> LDHLHAAEAAYQIESIIKTATDTVKSEINAELGVVPSLNAVETGATSNTEPEEAIQTRTVINQHGVSETLVENFLSRAALVSKRSFEYKDHTSSTARADKNFFKWTINTRSFVQLRRKLELFTYLRFDAEITILTTVAVNGSGNNTYVGLPDLTLQAMFVPTGALTPEKQDSFHWQSGSNASVFFKISDPPA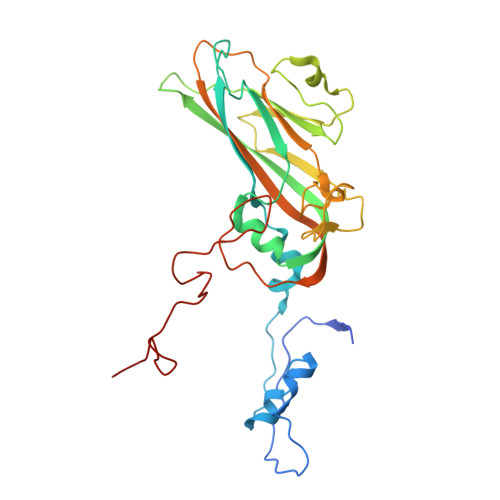RITIPFMCINSAYSVFYDGFAGFEKNGLYGINPADTIGNLCVRIVNEHQPVGFTVTVRVYMKPKHIKAWAPRPPRTLPYMSIANANYKGKERAPNALSAIIGNRDSVKTMPHNIVNT> MLKYKEILETIIE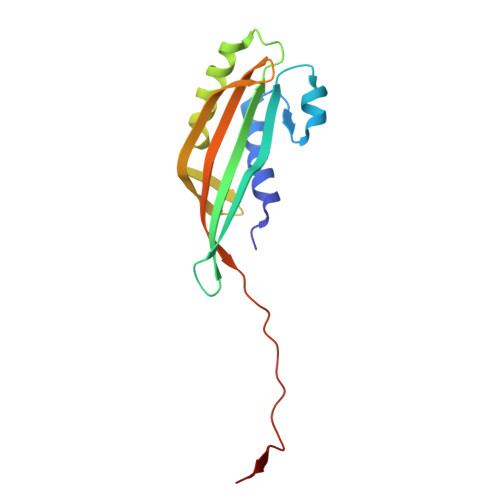ILKKNFTESIFIDDESVQGSEGSCFFVSILSVICTPVMLNTNNKDIVISIKYLPKPQSKSIRMYEISDELNKLFNRNIKVTDRKLNITKLEQSIKKEESIYVLNFTFTLNYLDSVYEEDVVYENMKEINLNLGE>MSQNVLGGVLRACSMDPETGFYRDGHCRTGPRDTGSHVVCAEMTEAFLEYTKRQGNDLMTPRPEMDFPGLEPGDRWCLCAARWREAMEAGVAPPVVLAATSEAALK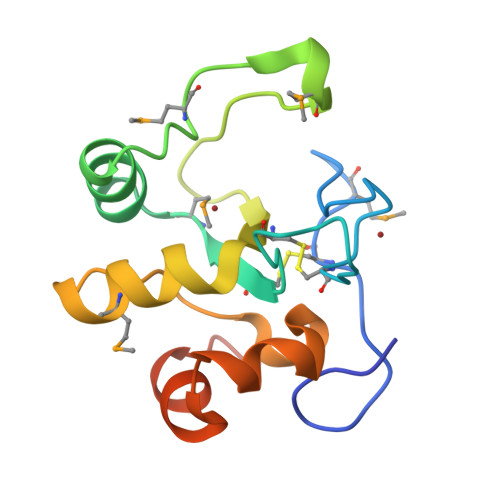AVDLEVLKAHAVDAPLEHHHHHH[2x]>[4x]MKLYIYDHCPYCLKARMIFGLKNIPVELHVLLNDDAETPTRMVGQKQVPILQKDDSRYMPESMDIVHYVDKLDGKPLLTGKRSPAIEEWLRK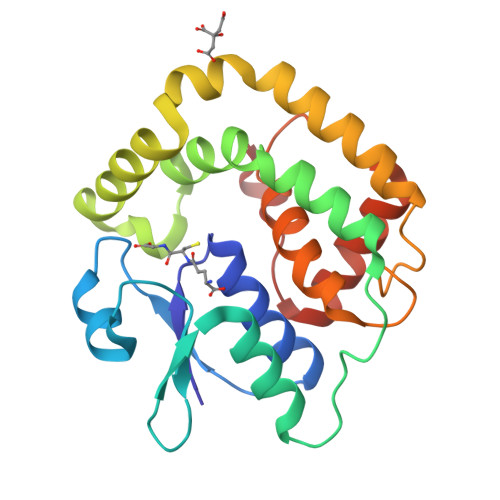VNGYANKLLLPRFAKSAFDEFSTPAARKYFVDKKEASAGNFADLLAHSDGLIKNISDDLRALDKLIVKPNAVNGELSEDDIQLFPLLRNLTLVAGINWPSRVADYRDNMAKQTQINLLSSMAI> AASEETLAFQRQLNALIGYDVTDVSNVHDDELEFTRRRLVTPRMAEVAGRDPKLYAMHPWVTSKPLPEYLLKKITNNCVFIVIHRSTTSQTIKVSADDTPGTILQSFFTKMAKKKSLMDIPESQNERDFVLRVCGRDEYLVGETPIKNFQWVRQCLKNGEEIHLVLDTPPDPALDEVRKEEWPLVDDCTGVTGYHEQLTIHGKDHESVFTVSLWDCDRKFRVKIRGIDIPVLPRTADLTVFVEANIQYGQQVLCQRRTSPKPFTEEVLWNVWLEFSIKIKDLPKGALLNLQIYCGAKPALSGKTSAEMPSPESKGKAQLLYYVNLLLIDHRFLLRHGEYVLHMWQLSGKGEDQGSFNADKLTSATNPDKENSMSISILLDNYCHPIALPKHRPTPDPEGDRVRAEMPNQLRKQLEAIIATDPLNPLTAEDKELLWHFRYESLKDPKAYPKLFSSVKWGQQEIVAKTYQLLAKREVWDQSALDVGLTMQLLDCNFSDENVRAIAVQKLESLEDDDVLHYLLQLVQAVKFEPYHDSALARFLLKRGLRNKRIGHFLFWFLRSEIAQSRHYQQRFAVILEAYLRGCGTAMLHDFTQQVQVIDMLQKVTIDIKSLSAEKYDVSSQVISQLKQKLENLQNLNLPQSFRVPYDPG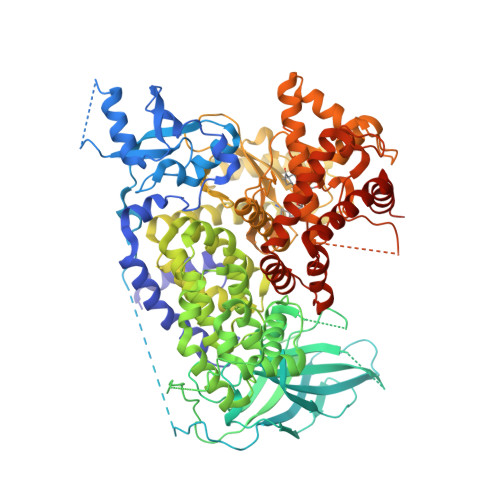LKAGALVIEKCKVMASKKKPLWLEFKCADPTALSNETIGIIFKHGDDLRQDMLILQILRIMESIWETESLDLCLLPYGCISTGDKIGMIEIVKDATTIAKIQQSTVGNTGAFKDEVLSHWLKEKCPIEEKFQAAVERFVYSCAGYCVATFVLGIGDRHNDNIMISETGNLFHIDFGHILGNYKSFLGINKERVPFVLTPDFLFVMGTSGKKTSLHFQKFQDVCVKAYLALRHHTNLLIILFSMMLMTGMPQLTSKEDIEYIRDALTVGKSEEDAKKYFLDQIEVCRDKGWTVQFNWFLHLVLGIKQGEKHSA>MVYKITVRVYQTNPDAFFHPVEKTVWKYA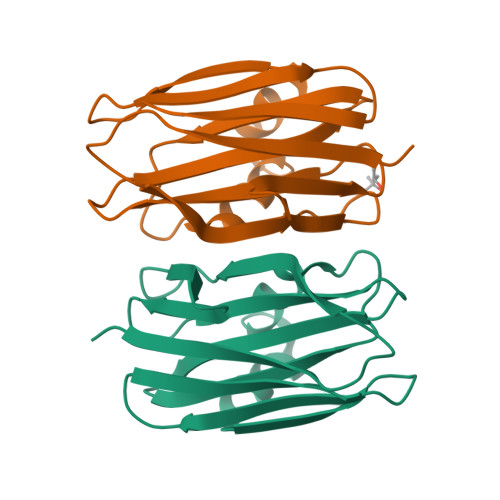NGGTWSITDDQHVLTMGGSGTSGTLRFHADNGESFTATFGVHNYKRWCDIVTNLAADETGMVINQQYYSQKNREEARERQLSNYQVKNAKGRNFQIVYTEAEGNDLHANLIIG[2x]> MIDIHSHIVFDVDDGPKSREESKALLAESYRQGVRTIVSTSHRRKGMFETPEEKIAENFLQVREIAKEVASDLVIAYGAEIYYTPDVLDKL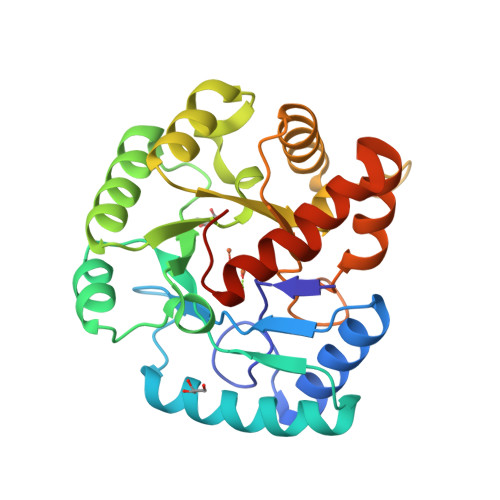EKKRIPTLNDSRYALIEFSMNTPYRDIHSALSKILMLGITPVIAHIERYDALENNEKRVRELIDMGCYTQVNSSHVLKPKLFGERYKFMKKRAQYFLEQDLVHVIASDMHNLDGRPPHMAEAYDLVTQKYGEAKAQELFIDNPRKIVMDQLILEHHHHHH>MLITKIVGHIDDYESSDKKVDWLEVEWEDLNKRILRKETENG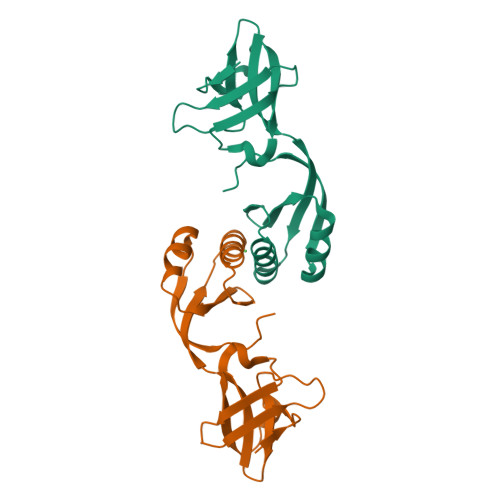TDIAIKLENSGTLRYGDVLYESDDTLIAIRTKLEKVYVIKPQTMQEMGKMAFEIGNRHTMCIIEDDEILVRYDKTLEKLIDEVGVSYEQSERRFKEPFKYRGHQH[2x]> NDVARGIVKADVAQNNFGLYGQGQIVAVADTGLDTGRNDSSMHEAFRGKITALYALGRTNNANDPNGHGTHVAGSVLGNATNKGMAPQANLVFQSIMDSGGGLGGLPANLQTLFSQAYSAGARIHTNSWGAPVNGAYTTDSRNVDDYVRKNDMTILFAAGNEGPGSGTISAPGTAKNAITVGATENLRPSFGSYADNINHVAQFSSRGPTRDGRIKPDVMAPGTYILSARSSLAPD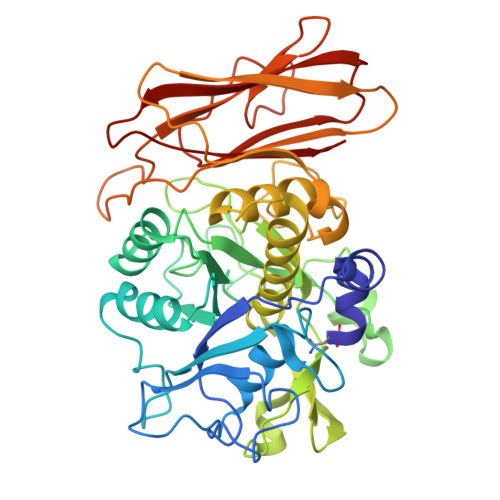SSFWANHDSKYAYMGGTSMATPIVAGNVAQLREHFVKNRGVTPKPSLLKAALIAGAADVGLGFPNGNQGWGRVTLDKSLNVAFVNETSPLSTSQKATYSFTAQAGKPLKISLVWSDAPGSTTASLTLVNDLDLVITAPNGTKYVGNDFTAPYDNNWDGRNNVENVFINAPQSGTYTVEVQAYNVPVGPQTFSLAIVH> MRLEFSIYRYNPDVDDAPRMQDYTLEADEGRDMMLLDALIQLKEKDPSLSFRRSCREGVCGSDGLNMNGKNGLACITPISALNQPGKKIVIRPLPGLPVIR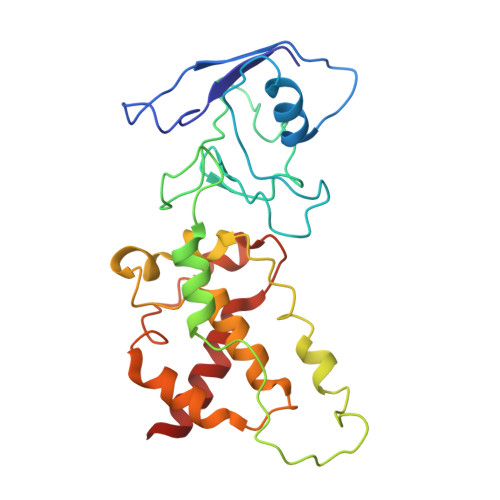DLVVDMGQFYAQYEKIKPYLLNNGQNPPAREHLQMPEQREKLDGLYECILCACCSTSCPSFWWNPDKFIGPAGLLAAYRFLIDSRDTETDSRLDGLSDAFSVFRCHSIMNCVSVCPKGLNPTRAIGHIKSMLLQRNA>[2x]MSLSESLAKYGITGATNIVHNPSHEELFAAETQASLEGFEKGTVTEMGAVNVMTGVYTGRSPKDKFIVKNEASKEIWWTSDEFKNDNKPVTEEAWAQLKALAGKELSNKPLYVVDLFCGANENTRLKIRFVMEVAWQAHFVTNMFIRPTEEELKGFEPDFVVLNASKAKVENFKELGLNSETAVVFNLAEKMQIILNTWYGGEMKKGMFSMMNFYLPLQGIAAMHCSANTDLEGKNTAIFFGLSGTGKTTLSTDPKRLLIGDDEHGWDDDGVFNFEGGCYAKVINLSKENEPDIWGAIKRNALLENVTVDANGKVDFADKSVTENTRVSYPIFHIKNIVKPVSKAPAAKRVIFLSADAFGVLPPVSILSKEQTKYYFLSGFTAKLAGTERGITEPTPTF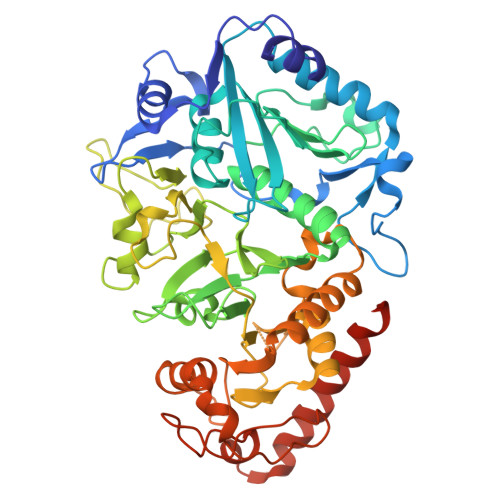SSCFGAAFLTLPPTKYAEVLVKRMEASGAKAYLVNTGWNGTGKRISIKDTRGIIDAILDGSIDTANTATIPYFNFTVPTELKGVDTKILDPRNTYADASEWEVKAKDLAERFQKNFKKFESLGGDLVKAGPQL BrlR, a member of the MerR family of multidrug efflux pump activators, consists of a structurally conserved N-terminal DNA-binding domain and a C-terminal GyrI-like binding domain. BrlR mediates the antibiotic resistance of P. aeruginosa by activating the expression of multidrug efflux pumps and repressing PhoPQ activation. The monomer can be divided into three domains: the N-terminal DNA-binding domain (residues 1–75), which adopts a winged helix-turn-helix fold; the long central α-helical linker (residues 76–119), which connects two terminal domains; and the C-terminal multidrug-binding domain (residues 120–270). Our most striking finding is that BrlR is not only a pyocyanin receptor but it is also a dual receptor that is responsive to both c-di-GMP and pyocyanin.

Despite great effort, we were unable to obtain diffraction-quality crystals of the BrlR-pyocyanin complex. The newly identified binding site is unique among those of all GyrI-like structures determined to date. The ligand is stabilized chiefly by hydrophobic interactions with the surrounding residues in addition to an H-bond with E247 at the bottom. The residues lining the pyocyanin binding pocket are conserved in many GyrI-like proteins, suggesting that the GyrI-like domains in other bacteria may also recognize pyocyanin. Together, the BrlR-C domain contains two adjacent binding sites within the multidrug-binding pocket. Hence, the pyocyanin binding pocket of BrlR-C domain is quite rigid. It is unlikely that the larger drug molecules located in the canonical binding pocket can slide into the pyocyanin binding site and promote BrlR-DNA binding, as reflected by the EMSA results for tobramycin. Among these ligands, pyocyanin is the only one expected to affect the interface of the two terminal domains in BrlR, and only the binding of pyocyanin to the corresponding site will induce a significant conformational change in the HTH motif.

>GSMHARIVERPAFSVVGMEYFGSAPGDTIGQLWERFIPREHEIAGKHDPEVSYGICAQQPNGEFHYVAGFEVQEGWPVPEGMVRFQVPAQKYAVFTHKGTAPQIAESFQAIYSHLLAERGLEPKAGVDFEYYDQRFRGPLDPNSQVDLYIPIY[2x]>[2x]VMKANVTKKTLNEGLGLLERVIPSRSSNPLLTALKVETSEGGLTLSGTNLEIDLSCFVPAEVQQPENFVVPAHLFAQIVRNLGGELVELELSGQELSVRSGGSDFKLQTGDIEAYPPLSFPAQADVSLDGGELSRAFSSVRYAASNEAFQAVFRGIKLEHHGESARVVASDGYRVAIRDFPASGDGKNLIIPARSVDELIRVLKDGEARFTYGDGMLTVTTDRVKMNLKLLDGD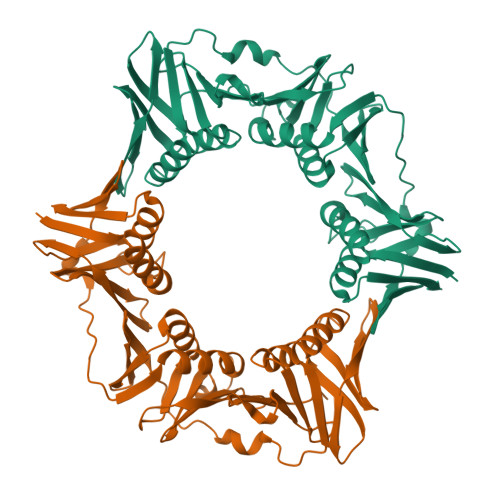FPDYERVIPKDIKLQVTLPATALKEAVNRVAVLADKNANNRVEFLVSEGTLRLAAEGDYGRAQDTLSVTQGGTEQAMSLAFNARHVLDALGPIDGDAELLFSGSTSPAIFRAVGGGGGYMAVMVTLRVENLYFQ>[2x]MGHHHHHHHHHHSSGHENLYFQGHMANRNVEKLASIDAQLRLLVPGKVSEDDKLVEYDALLLDKFLDILQDLHGEDLKEAVQQCYELSAEYEGKHDPKKLEELGSLLTSLDTGDSIVIAKAFSHMLNLANLAEELQIAYRRRIKLKSGDFADEANATTESDIEETFKRLVHKLNKSPEEVFDALKNQTVELVLTAHPTQSVRRSLLQKHGRIRNCLAQLYAKDITPDDKQELDEALHREIQAAFRTDEIRRTPPTPQDEMRAGMSYFHETIWKGVPKFLRRVDTALKNIGINERFPYNAPLIQFSSWMGGDRDGNPRVTPEVTRDVCLLARMMTSNMYFSQIEDLMIEMSMWRCNSELRVRAEELYRTARKDVKHYIEFWKRIPPNQPYRVILGDVRDKLYNTRERSRHLLVDGKS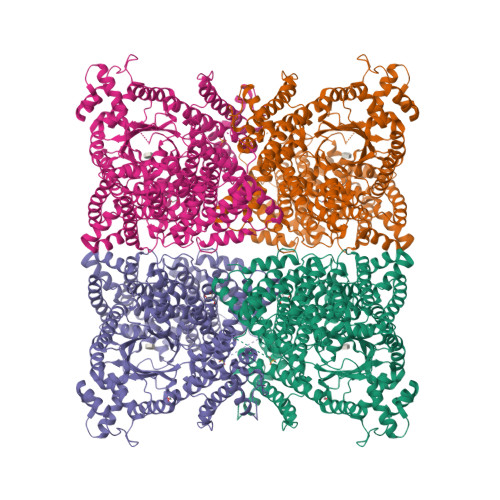DIPDEAVYTNVEQLLEPLELCYRSLCDCGDHVIADGSLLDFLRQVSTFGLSLVKLDIRQESDRHTEVLDAITQHLGIGSYREWSEEKRQEWLLAELSGKRPLIGPDLPKTEEVKDCLDTFKVLAELPSDCFGAYIISMATSTSDVLAVELLQREYHIKHPLRVVPLFEKLADLEAAPAAMTRLFSMDWYRNRIDGKQEVMIGYSDSGKDAGRFSAAWQLYKTQEQIVKIAKEFGVKLVIFHGRGGTVGRGGGPTHLALLSQPPDTINGSLRVTVQGEVIEQSFGEEHLCFRTLQRFCAATLEHGMNPPISPRPEWRELMDQMAVVATEEYRSVVFKEPRFVEYFRLATPELEFGRMNIGSRPSKRKPSGGIESLRAIPWIFSWTQTRFHLPVWLGFGAAFKHAIQKDSKNLQMLQEMYKTWPFFRVTIDLVEMVFAKGNPGIAALNDKLLVSEDLRPFGESLRANYEETKNYLLKIAGHKDLLEGDPYLKQGIRLRDPYITTLNVCQAYTLKRIRDPNYHVTLRPHISKEYAAEPSKPADELIHLNPTSEYAPGLEDTLILTMKGIAAGMQNTG> MNQNLLVTKRDGSTERINLDKIHRVLDWAAEGLHNVSISQVELRSHIQFYDGIKTSDIHETIIKAAADLISRDAPDYQYLAARLAIFHLRKKAYGQFEPPALYDHVVKMVEMGKYDNHLLEDYTEEEFKQMDTFIDHDRDMTFSYAAVKQLEGKYLVQNRVTGEIYESAQFLYILVAACLFSNYPRETRLQYVKRFYDAVSTFKISLPTPIMSGVRTPTRQFSSCVLIECGDSLDSINATSSAIVKYVSQRAGIGINAGRIRALGSPIRGGEAFHTGCIPFYKHFQTAVKSCSQGGVRGGAATLFYPMWHLEVESLLVLKNNRGVEGNRVRHMDYGVQINKLMYTRLLKGEDITLFSPSDVPGLYDAFFADQEEFERLYTKYEKDDSIRKQRVKAVELFSLMMQERASTGRIYIQNVDHCNTHSPFDPAIAPVRQSNLCLEIALPTKPLNDVNDENGEIALCTLSAFNLGAINNLDELEELAILAVRALDALLDYQDYPIPAAKRGAMGRRTLGIGVINFAYYLAKHGKRYSDGSANNLTHKTFEAIQYYLLKASNELAKEQGACPWFNETTYAKGILPIDTYKKDLDTIANEPLHYDWEALRESIKTHGLRNSTLSALMPSETSSQISNATNGIEPPRGYVSIKASKDGILRQVV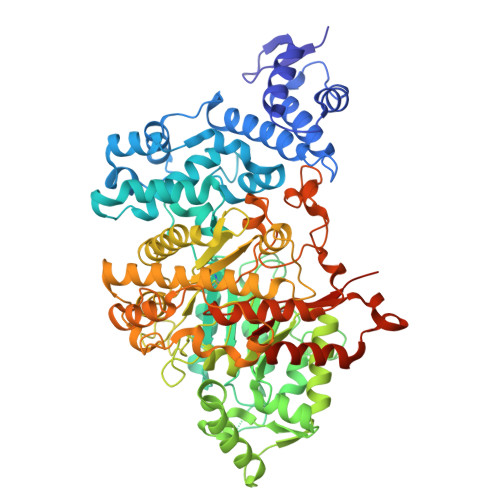PDYEHLHDAYELLWEMPGNDGYLQLVGIMQKFIDQSISANTNYDPSRFPSGKVPMQQLLKDLLTAYKFGVKTLYFQNTRDGAEDAQDDLVPSIQDDGCESGACKI> MQQRKKIYLRQKRKIYIQLKNKEKKKNNQFIQKREKMGYKIRNKSIFWTRAGWKNNWHPKNFNAPRPSYGEFTMGIRCRNDHHSFLRYVQTYRNMSRHCKQYFLGDKQLEETFILGLRSLFLVPYDSQCLTDQIKHGGERRFVDQLDRDFELISYNTHPYQLFTYTVRNEHLAWKNEQYEKIQKGEKTFEQELLDYLDEQVLAEKAKLRDGQNFSIERMTEIALHVFRKARAGKVRPAQDVRGPDGNVNDFLEQRRPFEHPNP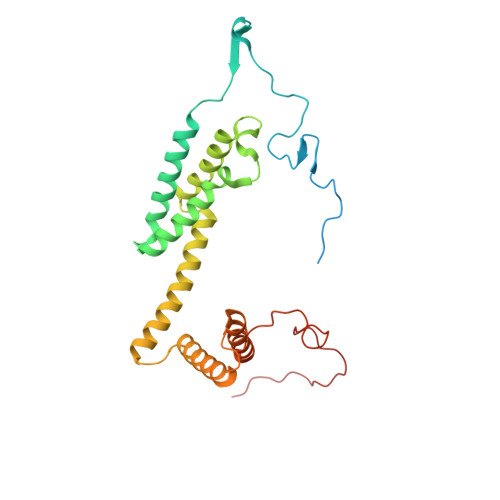TGVTH>SAAQPPWPQGGQIEFRDFGLRYRPELPLAVQGVSFKIHAGEKVGIVGRTGAGKSSLASGLLRLQ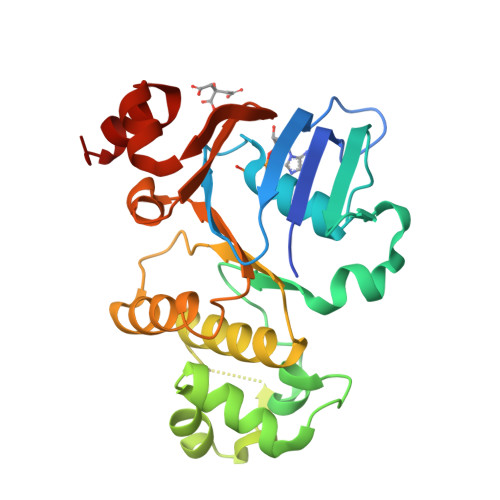EAAEGGIWIDGVPIAHVGLHTLRSRISIIPQDPILFPGSLRMNLDLLQEHSDEAIWAALETVQLKALVASLPGQLQYKCADRGEDLSVGQKQLLCLARALLRKTQILILDEATAAVDPGTELQMQAMLGSWFAQCTVLLIAHRLRSVMDCARVLVMDKGQVAESGSPAQLLAQKGLFYRLAQESGLV[2x]> MAAAMASAELQGKYQKLAQEYSKLRAQNQVLKKGVVDEQANSAALKEQLKMKDQSLRKLQQEMDSLTFRNLQLAKRVELLQDELALSEPRGKKNKKSGESSSQLSQEQKSVFDEDLQKKIEENERLHIQFFEADEQHKHVEAELRSRLATLETEAAQHQAVVDGLTRKYMETIEKLQNDKAKLEVKSQTLEKEAKECRLRTEECQLQLKTLHEDLSGRLEESLSIINEKVPFNDTKYSQYNALNVPLHNRRHQLKMRDIAGQALAFVQDLVTALLNFHTYTEQRIQIFPVDSAIDTISPLNQKFSQYLHENASYVRPLEEGMLHLFESITEDTVTVLETTVKLKTFSEHLTSYICFLRKILPYQLKSLEEECESSLCTSALRARNLELSQDMKKMTAVFEKLQTYIALLALPSTEPDGLLRTNYSSVLTNVGAALHGFHDVMKDISKHYSQKAAIEHELPTATQKLITTNDCILSSVVALTNGAGKIASFFSNNLDYFIASLSYGPKAASGFISPLSAECMLQYKKKAAAYMKSLRKPLLESVPYEEALANRRILLSSTESREGLAQQVQQSLEKISKLEQEKEHWMLEAQLAKIKLEKENQRIADKLKNTGSAQLVGLAQENAAVSNTAGQDEATAKAVLEPIQSTSLIGTLTRTSDSEVPDVESREDLIKNHYMARIVELTSQLQLADSKSVHFYAECRALSKRLALAEKSKEALTEEMKLASQNISRLQDELTTTKRSYEDQLS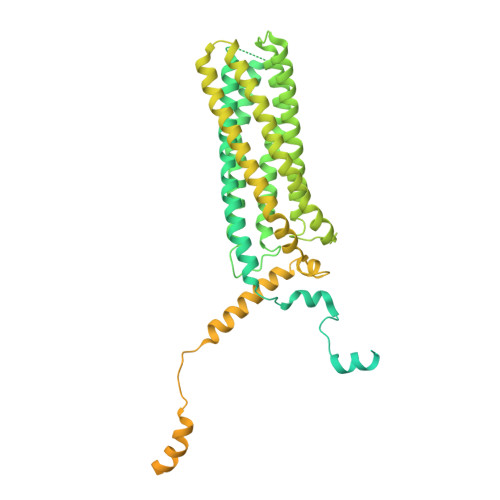MMSDHLCSMNETLSKQREEIDTLKMSSKGNSKKNKSR(3S)-1-{[(3,5-DIMETHYLISOXAZOL-4-YL)AMINO]CARBONYL}-4,4-DIMETHYLPYRROLIDIN-3-YL{(1S)-1-[1-HYDROXY-2-OXO-2-{[(1R)-1-PHENYLETHYL]AMINO}ETHYL]PENTYL}CARBAMATE 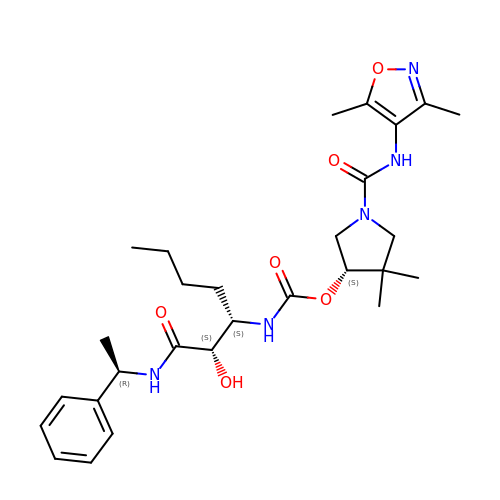| C28 H41 N5 O6 | VVZICJQTDYOKIN-TYVKFHQSSA-N>[2x]MNQQGFVISNELRQQQSELTSTWDLMLQTRINLSRSAARMMMDASNQQSSAKTDLLQNAKTTLAQAAAHYANFKNMTPLPAMAEASAN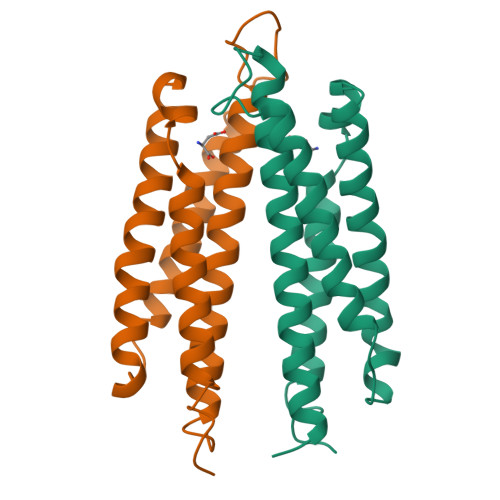VDEKYQRYQAALAELIQFLDNGNMDAYFAQPTQGMQNALGEALGNYARVSENLYRQTF> HVRSESSV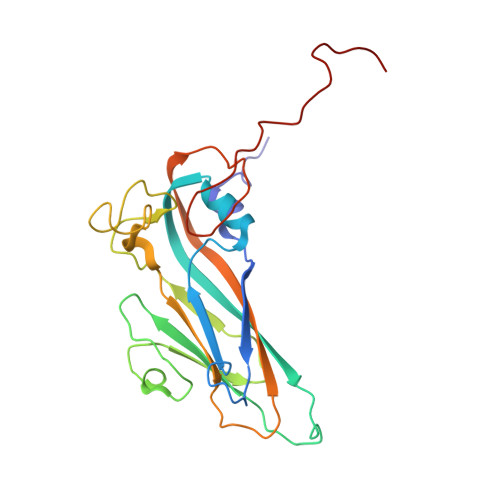ENFLSRSACVYIVEYKTRDDTPDKMYDSWVINTRQVAQLRRKLEFFTYVRFDVEVTFVITSVQDDSTRQNTDTPALTHQIMYVPPGGPIPQAVDDYNWQTSTNPSVFWTEGNAPPRMSIPFMSVGNAYSNFYDGWSHFSQTGVYGFNTLNNMGKLYFRHVNDKTISPITSKVRIYFKPKHVKAWVPRPPRLCEYTHKDNVDFEPKGVTTSRTQLTISNS>FHSGGVAECEGCHTMHNSLGGAVMNSATAQFTTGPMLLQGATQSSSCLNCHQHAGDTGPSSYHISTAEADMPAGTAPLQMTPGGDFGWVKKTYTWNVRGLNTSEGERKGHNIVAGDYNYVADTTLTTAPGGTYPANQLHCSSCHDPHGKYRRFVDGSIATTGLPIKNSGSYQNSNDPTAWGAVGAYRILGGTGYQPKSLSGSYAFANQVPAAVAPSTYNRTEATTQTRVAYGQGMSEWCANCHTDIHNSAYPTNLRHPAGNGAKFGATIAGLYNSYKKSGDLTGTQASAYLSLAPFEEGTADYTVLKGHAKIDDTALTGADATSNVNCLSCHRAHASGFDSMTRFNLAYEFTTIADASGN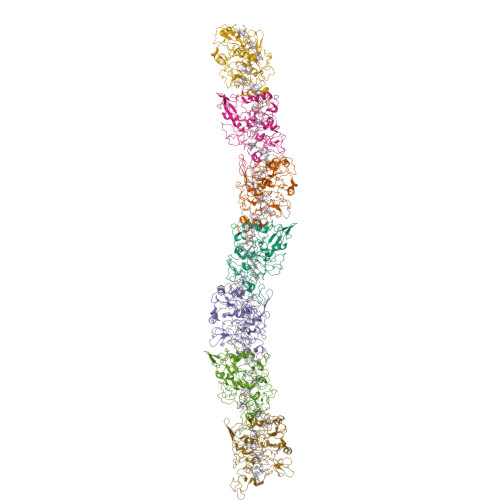SIYGTDPNTSSLQGRSVNEMTAAYYGRTADKFAPYQRALCNKCHAKD[7x]> MMNSIKFIFLGDVYGKAGRNIIKNNLAQLKSKYQADLVIVNAENTTHGKGLSLKHYEFLKEAGVNYITMGNHTWFQKLDLAVVINKKDLVRPLNLDTSFAFHNLGQGSLVFEFNKAKIRITNLLGTSVPLPFKTTNPFKVLKELILKRDCDLHIVDFHAETTSEKNAFCMAFDGYVTTIFGTHTHVPSADLRITP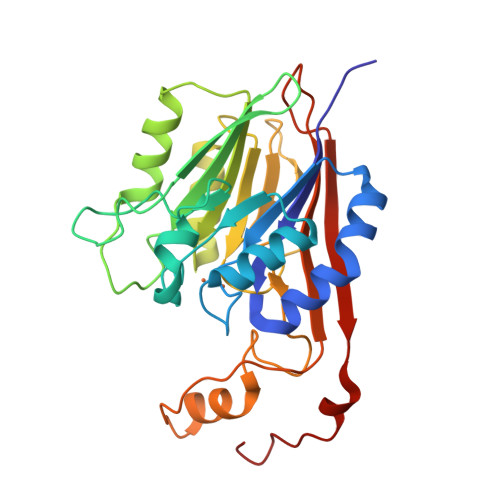KGSAYITDVGMCGPGFGSVIGANPEQSIRLFCAGSREHFEVSKCGAQLNGVFFEVDVNTKKVIKTEAIRIVEDDPRYLKQDYFNLI> QTSVSPSKVILPRGGSVLVTCSTSCDQPKLLGIETPLPKKELLLPGNNRKVYELSNVQEDSQPMCYSNCPDGQSTAKTFLTVYWTPERVELAPLPSWQPVGKNLTLRCQVEGGAPRANLTVVLLRGEKELKREPAVGEPAEVTTTVLVRRDHHGANFSCRTELDLRP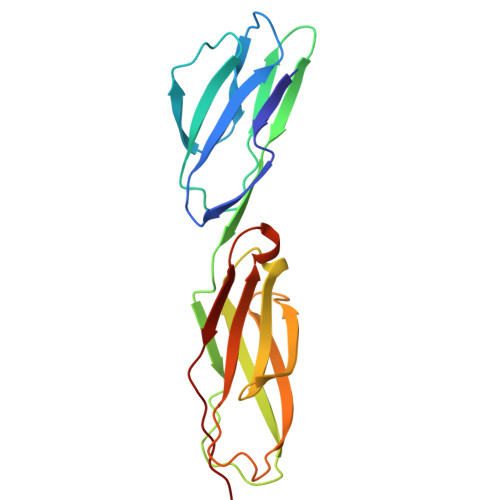QGLELFENTSAPYQLQTF>MSELILHHYPTSLFAEKARLMLGFKGVNWRSVTIPSIMPKPDLTALTG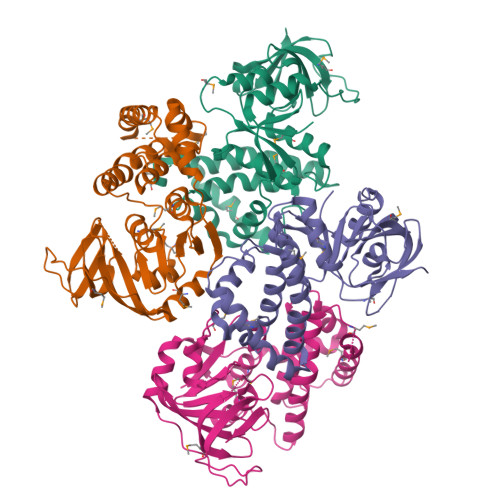GYRKTPVLQIGADIYCDTALMARRLEQEKASPAFYPQGQEFAVAGLAAWADSVLFLHAVSLVFQPESMAVRFAKVPPDAAKAFIADRSMLFNGGTASRPPVEQVKHQWPTFMSRLESQLSHGGDFLFGAPSIADFSVAHTLWFLKQTPVTAPFVDDYPSVSVWLDRVLGFGHGSLSDLSSAAAIEIASNATPAPLPDETFIDPNGFKAGDKVAIAAVDYGVEAVEGELMFTGREELILRREDNRAGVVHVHFPRLGFRVEKR[4x]>MRSNLLAFSIVASLGLAQVAHAAEGMWVPQQLPEIAGPLQKAGLKLSPEQLANLTGDPMGAVVALGGCTASFVSPQGLVVTNHHCAYGAIQLNSTAQKNLIKDGFNAPTLKDELSAGPNARVFVLDQITDVTAQAKAAIAGAGNDPLARSRALDAFDKAQVAACEADAGFRCRLYSFSGGNTYRLFRNMEIKDVRLVYAPPGSVGKFGGDVDNWMWPRHTGDFSFYRAYVGKDGKPAAFAADNVPYQPKHFLKFADQPLGADDFVMVAGYPGRTNRYALAGEFNETASFTYPTIAKHYNAVLKMIADAGKADADVKVKYAATAASMNNVAKNYLGQLEGFKRIDAAGQKQAEEAAVLAWLKKQGAAGKPALAAHAQLLKHLDTSKSTRERDLFVGQFNNTSAVGAAITLYRLSIERSKPDAEREAGYQERDLTTIEGGLKQMDRRYVAKMDQQLQTYWLDQYVALPAAQRDNEVLNKWLAGSDAAAVKSLVNKLGGTELGSLDTRLKWFKADRAAFEASNDPAIQYAVAVMPALLKQEEQKKIREGESLTARPLYLQAVADYKKSQGEFVYPDANLSLRITFGNVMGYGKDGVKYTPFTTLEGVAAKETGEDPFDSPKALLDAVKAKRYGGLEDKRLGSVPVNFLSNLDITGGNSGSPVLDANGKLVGLAFDGNWESVSSNWVFDPVMTRMIAVDSRYMQWIMQEVAPAPQLLKELNLAK[2x]

Family S46 peptidases are serine proteases showing dipeptidyl peptidase activity and are widely distributed in Bacteroidetes and Proteobacteria, but are not found in mammals. The SmDPP7 enzyme forms a homodimer, with each subunit consisting of 697 residues (Ala23-Ala719) and a molecular weight of approximately 155 kDa. Each subunit contains a catalytic double β-barrel domain harbouring the Asp-His-Ser catalytic triad (top domain) and an α-helical domain that caps the active site (bottom domain). SmDPP7 hydrolyses peptides from the N-terminus of oligopeptides, cleaving the dipeptide units (NH2-P2-P1-COOH) when the second P1 residue is a hydrophobic amino acid.

The unique features of the Val-Tyr complex are that the bottom space of the S2 subsite is occupied by four water molecules and the side chain of Lys206 is less ordered. In the Tyr-Tyr complex, one of the four water molecules at the bottom of the S2 subsite in the Val-Tyr complex is replaced by the hydroxy group of Tyr(P2) and the side chain of Lys206 is well ordered due to aliphatic contacts with the side chain of Tyr(P2). Because S46 peptidases involve conformational changes upon dipeptide binding, which reduce the degrees of freedom of the polypeptide chain, the transition from open to closed state is entropically unfavourable. For Val-Tyr, thermodynamic parameters were not determined due to low-avidity (Kd > 40 µM). The order of dissociation constants (Kd) of dipeptide (P2 a.a.; V > N > Y > L > F) was consistent with the result of competitive inhibition assay.>MFQQLSARLQEAIGRLRGRGRITEEDLKATLREIRRALMDADVNLEVARDFVERVREEALGKQVLESLTPAEVILATVYEALKEALGGEARLPVLKDRNLWFLVGLQGSGKTTTAAKLALYYKGKGRRPLLVAADTQRPAAREQLRLLGEKVGVPVLEVMDGESPESIRRRVEEKARLEARDLILVDTAGRLQIDEPLMGELARLKEVLGPDEVLLVLDAMTGQEALSVARAFDEKVGVTGLVLTKLDGDARGGAALSARHVTGKPIYFAGVSEKPEGLEPFYPERLAGRILGM[3x];>[3x]AIPWGGNLEEVLEELEMALLAADVGLSATEEILQEVRASGRKDLKEAVKEKLVGMLEPDERRATLRKLGFNPQKPKPVEPKGRVVLVVGVNGVGKTTTIAKLGRYYQNLGKKVMFCAGDTFRAAGGTQLSEWGKRLSIPVIQGPEGTDPAALAYDAVQAMKARGYDLLFVDTAGRLHTKHNLMEELKKVKRAIAKADPEEPKEVWLVLDAVTGQNGLEQAKKFHEAVGLT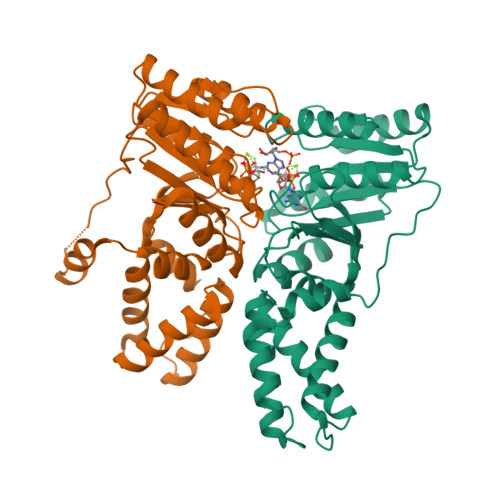GVIVTKLDGTAKGGVLIPIVRTLKVPIKFVGVGEGPDDLQPFDPEAFVEALLED>[2x]MLEGLSWVDYGERAELDDSDGHGNHRESSPFLSPLEASRGIDYYDRNLALFEEELDIRPKVSSLLGKLVSYTNLTQGAKEHEEAESGEGTRRRAAEAPSMGTLMGVYLPCLQNIFGVILFLRLTWMVGTAGVLQALLIVLICCCCTLLTAISMSAIATNGVVPAGGSYFMISRSLGPEFGGAVGLCFYLGTTFAAAMYILGAIEILLTYIAPPAAIFYPSGAHDTSNATLNNMRVYGTIFLTFMTLVVFVGVKYVNKFASLFLACVIISILSIYAGGIKSIFDPPVFPVCMLGNRTLSRDQFDICAKTAVVDNETVATQLWSFFCHSPNLTTDSCDPYFMLNNVTEIPGIPGAAAGVLQENLWSAYLEKGDIVEKHGLPSADAPSLKESLPLYVVADIATSFTVLVGIFFPSVTGIMAGSNRSGDLRDAQKSIPVGTILAIITTSLVYFSSVVLFGACIEGVVLRDKYGDGVSRNLVVGTLAWPSPWVIVIGSFFSTCGAGLQSLTGAPRLLQAIAKDNIIPFLRVFGHGKVNGEPTWALLLTALIAELGILIASLDMVAPILSMFFLMCYLFVNLACAVQTLLRTPNWRPRFKYYHWALSFLGMSLCLALMFVSSWYYALVAMLIAGMIYKYIEYQGAEKEWGDGIRGLSLSAARYALLRLEEGPPHTKNWRPQLLVLLKLDEDLHVKYPRLLTFASQLKAGKGLTIVGSVIQGSFLESYGEAQAAEQTIKNMMEIEKVKGFCQVVVASKVREGLAHLIQSCGLGGMRHNSVVLGWPYGWRQSEDPRAWKTFIDTVRCTTAAHLALLVPKNIAFYPSNHERYLEGHIDVWWIVHDGGMLMLLPFLLRQHKVWRKCRMRIFTVAQMDDNSIQMKKDLAVFLYHLRLEAEVEVVEMHNSDISAYTYERTLMMEQRSQMLRQMRLTKTEREREAQLVKDRHSALRLESLYSDEEDESAVGADKIQMTWTRDKYMTETWDPSHAPDNFRELVHIKPDQSNVRRMHTAVKLNEVIVTRSHDARLVLLNMPGPPRNSEGDENYMEFLEVLTEGLERVLLVRGGGREVITIYSAENLYFQ

Potassium‐coupled chloride transporters (KCCs) play crucial roles in regulating cell volume and intracellular chloride concentration. They are characteristically inhibited under isotonic conditions via phospho‐regulatory sites located within the cytoplasmic termini. Decreased inhibitory phosphorylation in response to hypotonic cell swelling stimulates transport activity, and dysfunction of this regulatory process has been associated with various human diseases. Here, we present cryo‐EM structures of human KCC3b and KCC1, revealing structural determinants for phospho‐regulation in both N‐ and C‐termini.

To gain further insights into the structure KCCs in an activated, non‐phosphorylated state, we took advantage of an N‐terminally deleted variant of the closely related KCC1 transporter (KCC1Δ19) with deleted N‐terminal OSR‐1‐binding motif H/RFXV (residues 3‐6 in full‐length KCC1 (Austin et␣al, 2014)). In both structures, TM7 and the cytoplasmic halves of broken helices TM1a and TM6b of the core domain (coloured in orange for KCC3b in Fig EV1A inset) are peeled away from the scaffold domains (TM helices 3–5, 8–10 in wheat in Fig EV1A), locking the TMD monomers into inward‐open conformations (Fig EV1B and C). In line with an obstructed ion path, the KCC3b‐PM map does not show any densities for cations coordinated by highly conserved residues of the cation‐binding site: Y232, I148, P443 and T446 (Fig EV2E). This interpretation is further supported by density for a putative cation coordinated by the corresponding residues in the KCC1Δ19 structure without N‐terminally “plugged” ion access path (Fig EV2F). Inspection of the electron density in this region of the KCC1 map suggests that either ADP or ATP are bound to the Rossmann‐like fold formed by β‐strands β1, β2 and β4 and helices α1, α3, α4 of the KCC1 inner lobe. Combined dipole charges from the converging N‐terminal ends of the three helices and multiple side chains create a positively charged nucleotide‐binding pocket (Fig 5B and Appendix␣Fig S10A). Weaker density for the γ‐phosphate indicates that a mixture of ADP‐ and ATP‐bound particles may contribute the observed densities (Fig EV4A). LC‐MS analysis of denatured purified KCC1 protein confirmed the presence of ADP and ATP in the sample (Appendix␣Fig S11), nucleotides that are likely carried along from the cell lysate during purification, or introduced by the ATP/MgCl2 wash step.>MPEGPELHLASQFVNEACRALVFGGCVEKSSVSRNPEVPFESSAYRISASARGKELRLILSPLPGAQPQQEPLALVFRFGMSGSFQLVPREELPRHAHLRFYTAPPGPRLALCFVDIRRFGRWDLGGKWQPGRGPCVLQEYQQFRENVLRNLADKAFDRPICEALLDQRFFNGIGNYLRAEILYRLKIPPFEKARSVLEALQQHRPSPELTLSQKIRTKLQNPDLLELCHSVPKEVVQLGGRGYGSESGEEDFAAFRAWLRCYGMPGMSSLQDR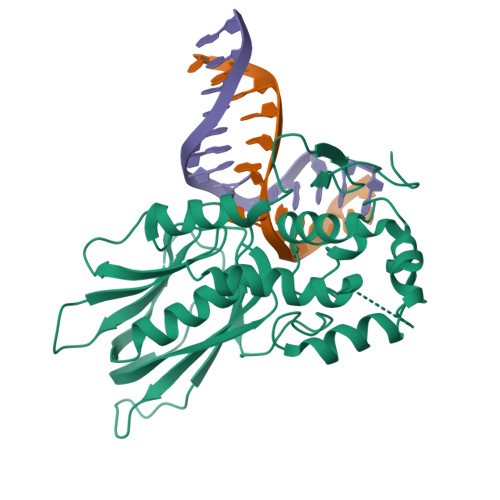HGRTIWFQGDPGPLAPKGRKS[3x]The pneumococcal serine-rich repeat protein (PsrP) is an important lung-specific virulence factor that is present in 60% of strains capable of causing pneumonia in children. Pneumococcal PsrP promotes both biofilm formation through self-oligomerization and adherence to keratin 10 (KRT10)-expressing lung epithelial cells. In this study, the crystal structure of the KRT10-binding region of PsrP (BR187–385) was determined, revealing a novel fold distantly related to CnaA subdomains. While one face of the compressed, two-sided barrel of BR187–385 is created by an extended β-sheet that presents a highly basic binding groove, extensive well-ordered loop regions distort the other face of the barrel, forming a paperclip-like substructure.

BR187–385 crystallized in two crystal forms of the space groups P43212 and P4122, with differing unit cell parameters. The native P4122 dataset that diffracted to 2.0 Å was solved using BR187–385 from P43212 as a template for molecular replacement (MR). A single BR187–385 molecule was found in the P4122 asymmetric unit, and a model comprising residues L203–S378 was refined to R- and Rfree-values of 17.7% and 20.1%, respectively. The structural deviation between the P4122-BR187–385 monomer and each of the three P43212-BR187–385 molecules was minimal, with root mean square deviations (r.m.s.d.) of 0.6 Å and less than 0.4 Å, following superposition of the P4122 monomer on the P43212 chains A and B/C, respectively. Crystal packing analysis revealed that two symmetry-related molecules in the P4122 crystal formed an intermolecular β-sheet resulting in an interface area of 585 Å2. However, a single population with a sedimentation coefficient of 1.85 S corresponding to a monomer with a hydrodynamic radius of 25 Å was clearly assessed using analytical ultracentrifugation (AUC). We believe, at the present stage, that the formed pseudo-complexes are probably owing to crystal packing. The overall three-dimensional structure of BR187–385, composed of 43% β-strands, 2% α-helices, 17% turns and 38% loop regions, can be described as a compressed barrel with two remarkably different faces. Furthermore, inspection of the electrostatic surface of BR187–385 revealed the presence of a highly basic groove with a solvent-accessible surface area of 180 Å2 that could easily accommodate the elongated and negatively charged helical rod domain of KRT10. A substructure within this region takes a paperclip form with back- and front-loops formed by residues 268–295 and 305–324, respectively, which provides a possible explanation to previous experimental observations.

> HHHHHHSGNTIVNGAPAINASLNIAKSETKVYTGEGVDSVYRVPIYYKLKVTNDGSKLTFTYTVTYVNPKTNDLGNISSMRPGYSIYNSGTSTQTMLTLGSDLGKPSGVKNYITDKNGRQVLSYNTSTMTTQGSGYTWGNGAQMNGFFAKKGYGLTSSWTVPITGTDTSFTFTPYAARTDRIGINYFNGGGKVVESSTTSQSLSQ> EPQYEE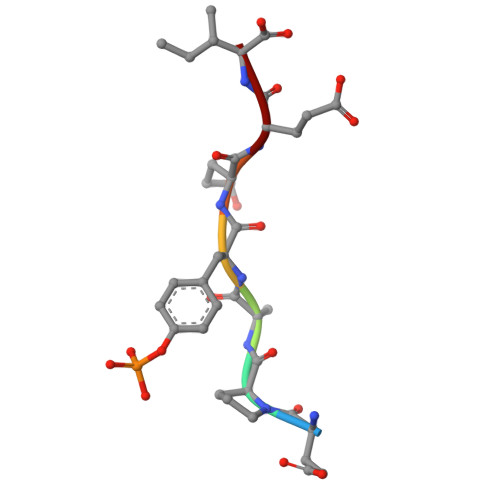I>[2x]SNAME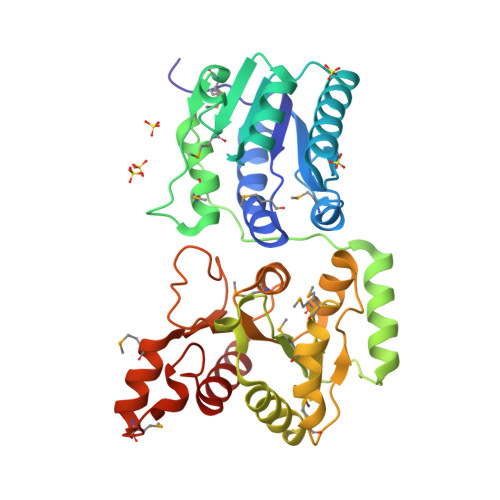LDYKRIVVTFLMHLGDVILTTPFLEVLRKAAPHSHITYVIDEKLQQVMEYNPNIDELIVVDKKGRHNSISGLNEVAREINAKGKTDIVINLHPNERTSYLAWKIHAPITTGMSHFLFRPFMTKYTRLDRKTRHAADMYINVLEQLGVTDTSNSGLHIEICEEWRCQAQEFYSSHGLTDTDILIGFNIGSAVPEKRWPAERFAHVADYFGRLGYKTVFFGGPMDLEMVQPVVEQMETKPIVATGKFQLGPLAAAMNRCNLLITNDSGPMHVGISQGVPIVALYGPSNPFFYGPYQAHAIVLETMDSYEIGKSMKKIIKEGNYKGLSVISEEQVIKAAETLLLESK Octopine dehydrogenase (OcDH, N2-(D-1-carboxyethyl)-L-arginine:NAD+-oxidoreductase, EC 1.5.1.11) catalyzes the reductive condensation of L-arginine and pyruvate in the presence of NADH to yield D-octopine [(R)-N2-(1-carboxyethyl)-L-arginine], NAD+, and water. The enzyme consists of two domains, an NADH binding domain and a so-called octopine-binding domain. Furthermore, a catalytic dyad comprising a His–Asp proton relay system and an additional Arg-sensor (Arg324) were identified. In summary, substrates of OcDH bind in an ordered sequential manner.

The evaluation of the data clearly demonstrates that agmatine acts as a competitive inhibitor with a Ki of 40±2 mM. Since no sequence assignment could be established in the NMR experiments, we solved the structure of the OcDH/NADH-Agmatine complex by X-ray crystallography. A 2.8 Å dataset was collected and initial phases were obtained by a rigid body refinement with the OcDH/NADH-pyruvate structure as template. Already during the initial round of refinement after rigid body refinement and manual building it became obvious that agmatine is bound inside the structure in a fashion similar to L-arginine in the OcDH/NADH-L-arginine complex. The guanidinium headgroup of agmatine is coordinated via interactions with the side chains of Glu142 (domain I) and Trp278 (domain II) as well as backbone interactions with Met206 (domain II). The Cβ atom is bound via backbone interactions of Ser207. However, the binding of agmatine induces a similar rotational movement of domain II towards domain I, which is almost identical to the domain closure observed in the OcDH/NADH-L-arginine structure. This is reflected in the RMSD value between the L-arginine and agmatine structure is 0.6 Å over 399 Cα atoms whereas the comparison with OcDH/NADH complex is 1.5 Å over 399 Cα atoms. Also the structure of the OcDH/NADH-agmatine complex indicates that the binding of the L-arginine side chain triggers the domain closure of OcDH and not the carboxyl moiety of the amino acids, a prerequisite for catalyzing octopine synthesis by OcDH.

> MTVKVCVCGGGNGAHTLSGLAASRDGVEVRVLTLFADEAERWTKALGADELTVIVNEKDGTQTEVKSRPKVITKDPEIAISGADVVILTVPAFAHEGYFQAMAPYVQDSALIVGLPSQAGFEFQCRDILGDKAAAVSMMSFETLPWACRIKEFGRKVEVLGTKSVLAASLIKGTAKTVDPLSTLQMLHGAEPVFRLAKHFLEMLIMSYSFVHPAILFGRWGSWDGKPVPEAPLFYQGIDQATADMLTACSNECKDVANAIMAACPGNDLSDDKDIYQWYLEYYHEDIQDDHDLYHAITTNKSYKGLVHPVKAVDAGVAPDFGNRYLTEDIPMGMIVFKGVAIAAGVAIPSNDKLIMWAQEKIGKEYLVDGALTGKDVATTRCPQRYGFNTLDAILTGKKHHHHH> MAQAPEYHYVGSVDYQPTRPSAHQ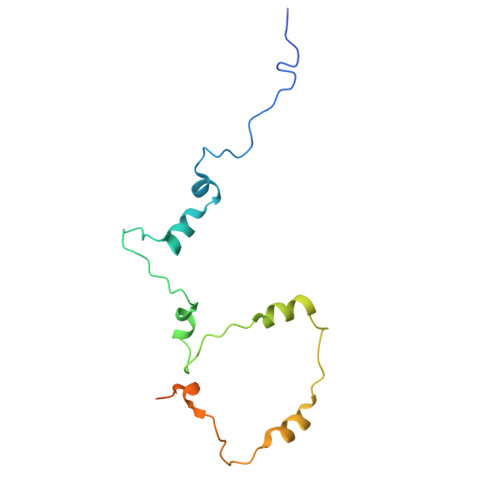NLIELYGLTELAKKVGRVDEFGNKRKMRRSYKAYIQDLPGYNEILRDNTIKQWLTNPIREEVPIDIEFLHHVFSVEPGIIPGFNPKVFGLEDDVVMGNVSRDSSQPRSPSRRKK>[3x]GPDSMTSENPDVLLSRVINVVRAASSLASQDVDFYKNLDRGFSKDLKSKADKLADMANEIILSIDEHHESFELKEEDISDLWNNFGNIMDNLLEMSDHSLDKLNCAINSKSRGSD;>MEDIEKIKPYVRSFSKALDELKPEIEKLTSKSLDEQLLLLSDERAKLELINRYAYVLSSLMFANMKVLGVKDMSPILGELKRVKSYMDKAKQYDNRITK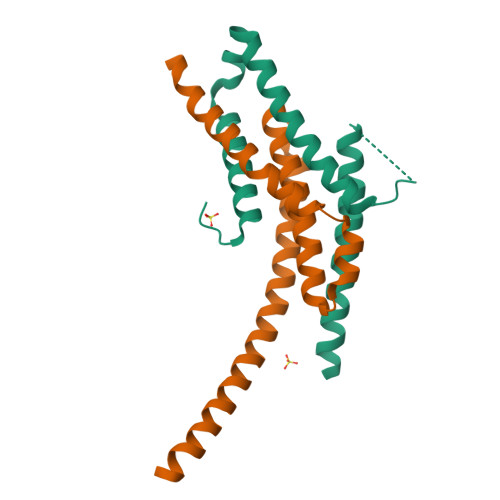SNEKSQAEQEKAKNIISNVLDGNKNQFEPSISRS[3x]> MADPTPVSVSGGTIHFEGKLVNAACAVSTKSADQTVTLGQYRTASFTAIGDTTAQVPFSIVLNDCDPKVAATAAVAFSGQADNTNTNLLAVSSADNSTTATGVGIEILDN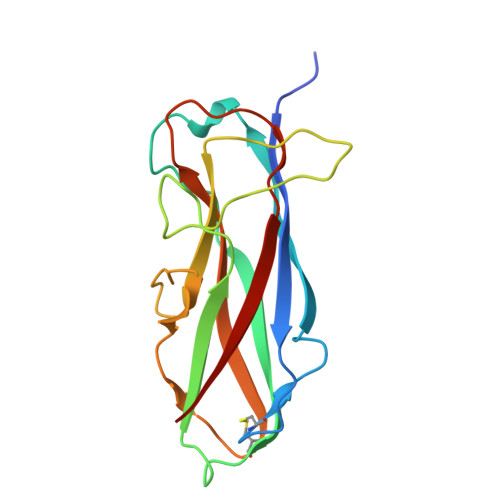TSSPLKPDGATFSAKQALVEGTNTLRFTARYKATAAATTPGQANADATFIMKYE> MMEKPEGLKLIDENGRRIDGRKKYELRPIKMEVGVLKNANGSAYIEWGKNKIIAAVYGPRELHPKHLQRPDRAILRVRYNMAPFSVEERKKPGPDRRSIEISKVIKGALEPALILEMFPRTAIDVFIEVLQADAGTRVAGITAASLALADAGIPMRDLVAACAAGKIEGEIV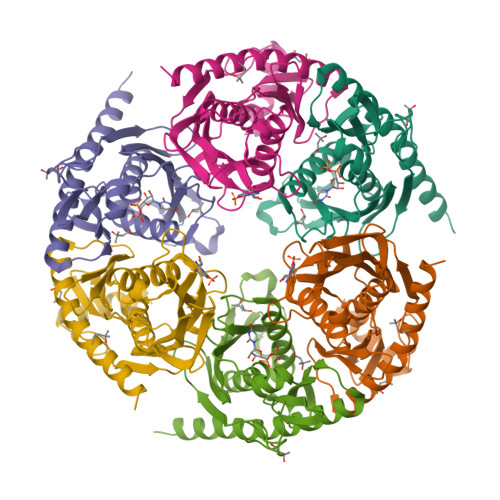LDLNKEEDNYGEADVPVAIMPLKNDITLLQMDGYLTKDEFIEAVKLAIKGAKAVYQKQREALKEKYLKIAQEVEGSE;> GSHMSDNEIVAGIMRDHIINLLKEGKRIDDRGFEDYRPIEIEVGVIEKAEGSALVKLGSTQVLVGIKTSLGEPFPDTPNMGVMTTNVELVPLASPTFEPGPPDERAIELARVIDRGIRESKALNLEKMVIVPGKIVRVVFIDVHVLDHDGNLMDAIGIAAIAALLNARVPKVRYNEETGEVETLDETEPLPVEKIPVPVTFAKIGNILVVDPSLDEELVMDGKITITTDETGHISAVQKSEGGAFKLEEVMYAVETAFKKAEEIRKLILEAVEKAKQ N-(6-aminohexanoyl)-3-methyl-L-valyl-3-methyl-L-valyl-N~1~-[(2S,3S)-3-hydroxy-4-oxo-4-{[(1R)-1-phenylpropyl]amino}butan-2-yl]-N~4~,N~4~-dimethyl-L-aspartamide | C37 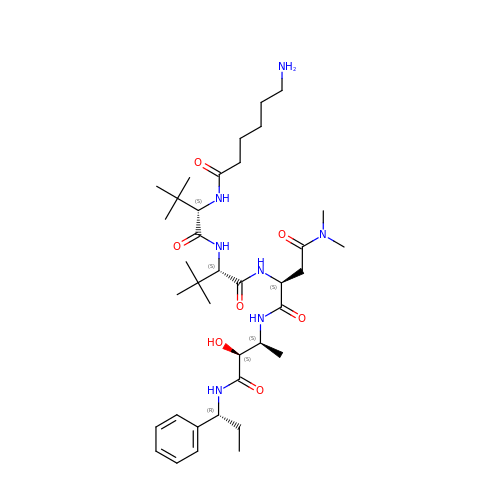H63 N7 O7 | RICYNZHPHSJRNO-GYZAPQSVSA-N>SWVWNQMFVLEEFSGPEPILVGRLHTDLDPGSKKIKYILSGDGAGTIFQINDITGDIHAIKRLDREEKAEYTLTAQAVD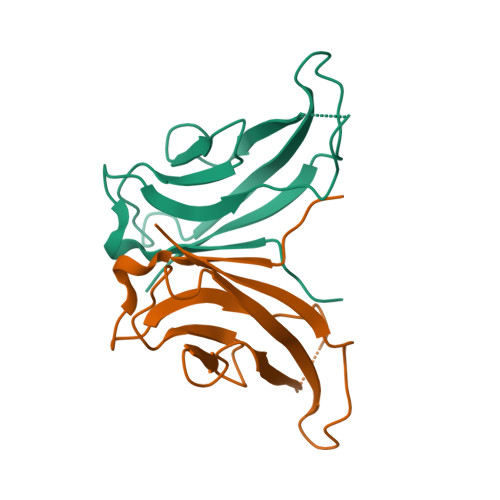FETNKPLEPPSEFIIKVQD[2x]> GTSSMADIGSELGFNEAERQKILDSNSSLMGNANEVRDKFIQNYASSLKDSNDP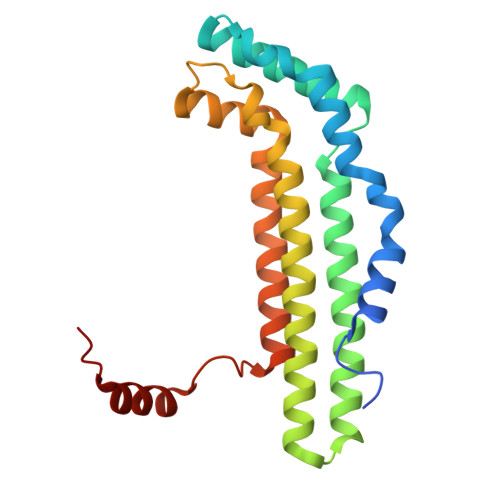QDFLRRVQELRINMQKNFISFDVYYNYLNNLVLASYNRCKQEKTFAESTIKNELTLGEFVAEISDNFNNFMCDEVARISDLVASYLPREYLPPFIDGNMMGVAFQILGIDDFGRKLNEIVQDIGTKYIILSKNKTYLTSLERAKLITQLKLNLE> ELPDFFQGKHFFLYGEFPGDERRKLIRYVTAFNGELEDYMSDRVQ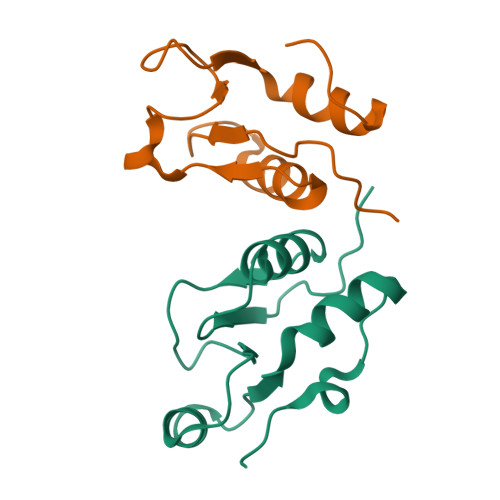FVITAQEWDPSFEEALMDNPSLAFVRPRWIYSCNEKQKLLPHQLYGVVPQA;> KVLLDIFTGVRLYLPPSTPDFSRLRRYFVAFDGDLVQEFDMTSATHVLGSRDKNPAAQQVSPEWIWACIRKRRLVAPS> MKSHKMMGGGISMHYITACLKIISD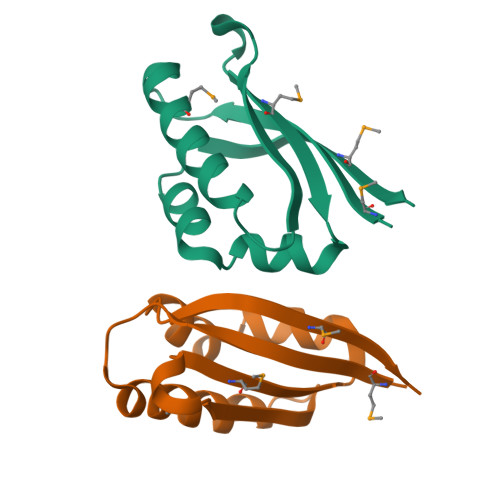KDLNEIMKEFKKLEEETNKEEGCITFHAYPLEPSERKIMLWEIWENEEAVKIHFTKKHTIDVQKQELTEVEWLMKSNVND> GPLG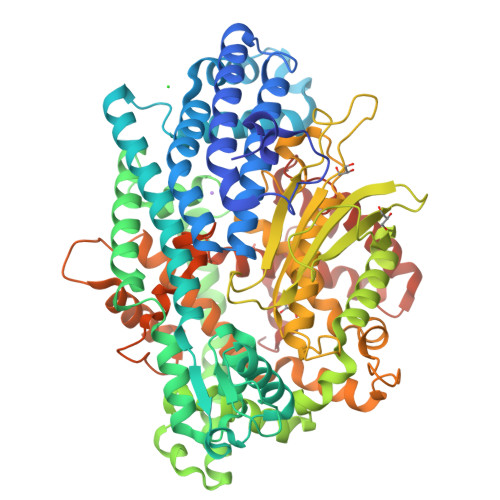SAAAVESVVSDETLSSNPLLQDFDFPPFDSVDASHVRPGIRALLQHLEAELEELEKSVEPTWPKLVEPLEKIVDRLTVVWGMINHLKAVKDTPELRAAIEDVQPEKVKFQLRLGQSKPIYNAFKAIRESPDWSSLSEARQRLVEAQIKEAVLIGIALDDEKREEFNKIEQELEKLSHKFSENVLDATKKFEKLITDKKEIEGLPPSALGLFAQAAVSKGHENATAENGPWIITLDAPSYLPVMQHAKNRALREEVYRAYLSRASSGDLDNTAIIDQILKLRLEKAKLLGYNNYAEVSMAMKMATVEKAAELLEKLRSASWDAAVQDMEDLKSFAKNQGAAESDSMTHWDTTFWSERLRESKYDINEEELRPYFSLPKVMDGLFSLAKTLFGIDIEPADGLAPVWNNDVRFYRVKDSSGNPIAYFYFDPYSRPSEKRGGAWMDEVVSRSRVMAQKGSSVRLPVAHMVCNQTPPVGDKPSLMTFREVETVFHEFGHALQHMLTKQDEGLVAGIRNIEWDAVELPSQFMENWCYHRDTLMSIAKHYETGETLPEEVYKKLLAARTFRAGSFSLRQLKFASVDLELHTKYVPGGPESIYDVDQRVSVKTQVIPPLPEDRFLCSFSHIFAGGYAAGYYSYKWAEVLSADAFSAFEDAGLDDIKAVKETGQRFRNTILALGGGKAPLKVFVEFRGREPSPEPLLRHNGLLAASASA>MRGSHHHHHHGSLSSSPSEILQELGKGSTHPQPGVSPPAAPAAPGPKDGPGETDAFGNSEGKELVASGENKIKQGLLPSLEDLLFYTIAEGQEKIPVHKFITALKSTGLRTSDPRLKECMDMLRLTLQTTSDGVMLDKDLFKKCVQSNIVLLTQAFRRKFVIPDFMSFTSHIDELYESAKKQSGGKVADYIPQLAKFSPDLWGVSVCTADGQRHSTGDTKVPFCLQSCVKPLKYAIAVNDLGTEYVHRYVGKEPSGLRFNKLFLNEDDKPHNPMVNAGAIVVTSLIKQGVNNAEKFDYVMQFLNKMAGNEYVGFSNATFQSERESGDRNFAIGYYLKEKKCFPEGTDMVGILDFYFQLCSIEVTCESASVMAATLANGGFCPITGERVLSPEAVRNTLSLMHSCGMYDFSGQFAFHVGLPAKSGVAGGILLVVPNVMGMMCWSPPLDKMGNSVKGIHFCHDLVSLCNFHNYDNLRHFAKKLDPRREGGDQRHSFGPLDYESLQQELALKETVWKKVSPESNEDISTTVVYRMESLGEKS[3x];> MRGSHHHHHHGSLSSSPSEILQELGKGSTHPQPGVSPPAAPAAPGPKDGPGETDAFGNSEGKELVASGENKIKQGLLPSLEDLLFYTIAEGQEKIPVHKFITALKSTGLRTSDPRLKECMDMLRLTLQTTSDGVMLDKDLFKKCVNSNIVLLTQAFRRKFVIPDFMSFTSHIDELYESAKKQSGGKVADYIPQLAKFSPDLWGVSVCTADGQRHSTGDTKVPFCLQSCVKPLKYAIAVNDLGTEYVHRYVGKEPSGLRFNKLFLNEDDKPHNPMVNAGAIVVTSLIKQGVNNAEKFDYVMQFLNKMAGNEYVGFSNATFQSERESGDRNFAIGYYLKEKKCFPEGTDMVGILDFYFQLCSIEVTCESASVMAATLANGG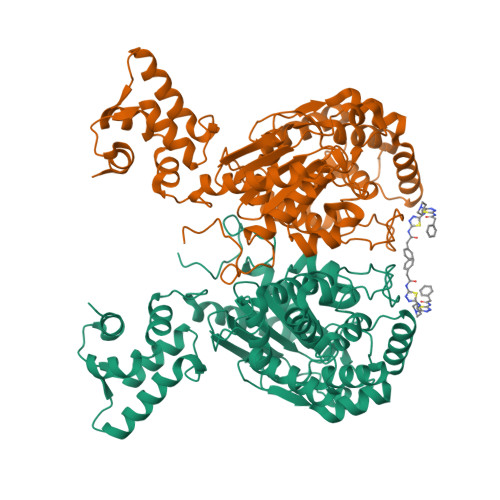FCPITGERVLSPEAVRNTLSLMHSCGMYDFSGQFAFHVGLPAKSGVAGGILLVVPNVMGMMCWSPPLDKMGNSVKGIHFCHDLVSLCNFHNYDNLRHFAKKLDPRREGGDQRHSFGPLDYESLQQELALKETVWKKVSPESNEDISTTVVYRMESLGEKS>MFQGSIVALITPFKEGEVDYEALGNLIEFHVDNGTDAILVCGTTGESPTLTFEEHEKVIEFAVKRAAGRIKVIAGTGGNATHEAVHLTAHAKEVGADGALVVVPYYNKPTQRGLYEHFKTVAQEVDIPIIIYNIPSRTCVEISVDTMFKLASECENIVASKESTPN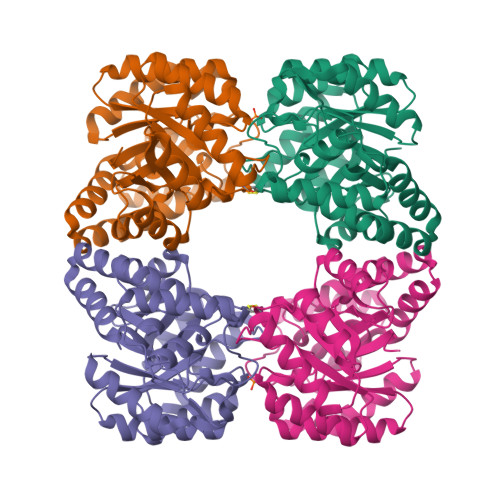MDRISEIVKRLGESFSVLSGDDSLTLPMMALGAKGVISVANNVMPREVKELIRAALEGDFRRAREIHYYLHDLFKVLFIETNPIPVKTACWMLGMCEKEFRLPLTEMSPENENKLREVLKKYNLPLKN[4x]>SENVSLNNISMQILRELLQYRRHLTDPVKNSAKEEEIIKTVQLPRIEYFIKNKKPIEFILPAFPTKSPNINKVLGTAPDMAERLSLIFLNSFCQRIQLYYPPGARIIICSDGHVFGDLIHVSDEVISQYHEDIKQLLHEVGAINLSTFNLNDDKELCEHSDDFNLQRQMLV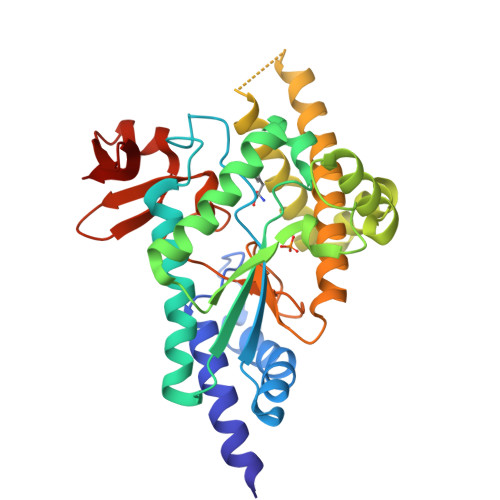KHYARSEASIKDELLQNNNGLQLYRAVTRFLYEDSLLPGYTGSNNALQKDAKQRAIGVIQRSWAWGSLLDTHFPKAIRLSIHPQPADSIKFGIHMMPTRDDWLTPWHGVAANVNGQFILMKHKEVQMMGGKLVNIHGKPSHYVI[2x]> MADSPNRLNRAKIDSTTMKDPRVLNNLKLRELLLPKFTSLWEIQTEVTVDNRTILLTWMHLLCESFELDKSVFPLSVSILDRYLCKKQGTKKTLQKIGAACVLIGSKIRTVKPMTVSKLTYLSCDCFTNLELINQEKDILEALKWDTEAVLATDFLIPLCNALKIPEDLWPQLYEAASTTICKALIQPNIALLSPGLICAGGLLTTIETDNTNCRPWTCYLEDLSSILNFSTNTVRTVKDQVSEAFSLYDLEIL;> MEKDGLCRADQQYECVAEIGEGAYGKVFKARDLKNGGRFVALKRVRVQTGEEGMPLSTIREVAVLRHLETFEHPNVVRLFDVCTVSRTDRETKLTLV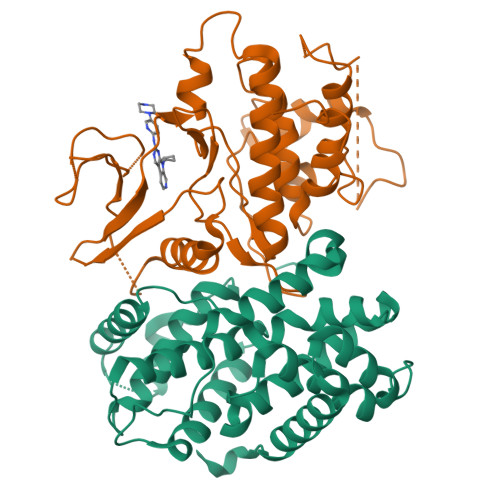FEHVDQDLTTYLDKVPEPGVPTETIKDMMFQLLRGLDFLHSHRVVHRDLKPQNILVTSSGQIKLADFGLARIYSFQMALTSVVVTLWYRAPEVLLQSSYATPVDLWSVGCIFAEMFRRKPLFRGSSDVDQLGKILDVIGLPGEEDWPRDVALPRQAFHSKSAQPIEKFVTDIDELGKDLLLKCLTFNPAKRISAYSALSHPYFQDLERCKENLDSHLPPSQNTSELNTA>[6x]EVYGIIAMQAAYRDYDSGDAKQDDNLGGMQLNNESRIGFRGKKQFANFEPTFIWQIEGGYVDPSFGGEGAGLGERDTFVGFESASWGQVRLGRVLTPMYELVDWPASNPGLGDVYDWGGAIGGAKYQDRQSNTIRWDSPMYADKFSIDAAVGAGDKAGLGAGDDYWGGIAAHYKLGPLQLDAAYEGNRNIEAEGQTW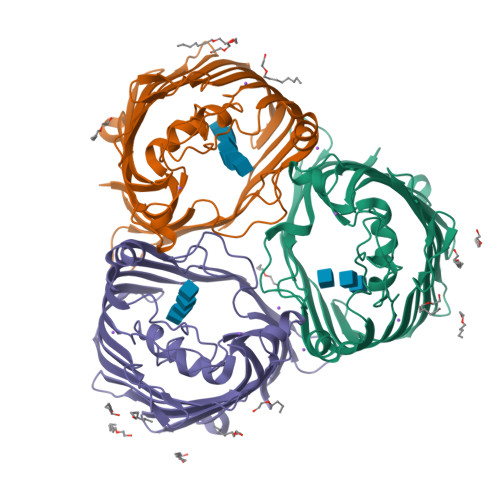ENNTYLVGVQGWFENGISFFAQYKYMEADASNGVNEKQDAMSAGLMYTTGDWQYKLGYAANFDLERDGKTLSNTSDDVVSAQIMYFVDPSAVLYARARMNDFNEGLDGLDDAARWTSGTNGDYNEYSVGVEYYF> MGSCCSCLKDSSDEASVSYLEDKDQLDFYSGGPLKALTTLVYSDNLNLQRSAALAFAEITEKYVRQVSREVLEPILILLQSQDPQIQVAAC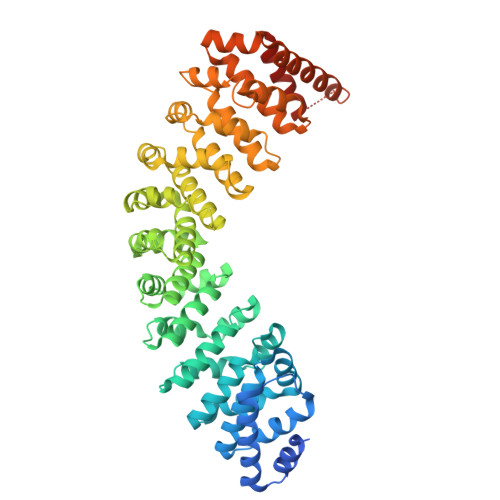AALGNLAVNNENKLLIVEMGGLEPLINQMMGDNVEVQCNAVGCITNLATRDDNKHKIATSGALIPLTKLAKSKHIRVQRNATGALLNMTHSEENRKELVNAGAVPVLVSLLSSTDPDVQYYCTTALSNIAVDEANRKKLAQTEPRLVSKLVSLMDSPSSRVKCQATLALRNLASDTSYQLEIVRAGGLPHLVKLIQSDSIPLVLASVACIRNISIHPLNEGLIVDAGFLKPLVRLLDYKDSEEIQCHAVSTLRNLAASSEKNRKEFFESGAVEKCKELALDSPVSVQSEISACFAILALADVSKLDLLEANILDALIPMTFSQNQEVSGNAAAALANLCSRVNNYTKIIEAWDRPNEGIRGFLIRFLKSDYATFEHIALWTILQLLESHNDKVEDLVKNDDDIINGVRKMADVTFERLQRSGIDVKNPGSNNNPSSNDNNSNNNDTGSEHQPVEDASLELYNITQQILQFLH2-{N'-[2-(5-AMINO-1-PHENYLCARBAMOYL-PENTYLCARBAMOYL)-HEXYL]-HYDRAZINOMETHYL}-HEXANOIC ACID(5-AMINO-1-PHENYLCARBAMOYL-PENTYL)-AMIDE | C38 H62 N8 O4 | 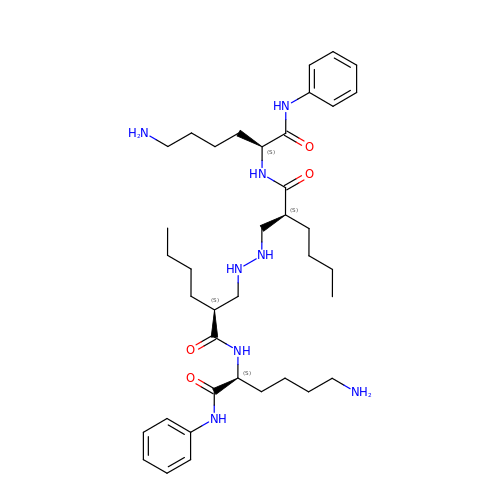YFMXWONORHSZEM-ANFUHZJESA-N> HTIFVQLEADGTTYPVSYGIRTPSYDGPITDVTSNDLACNGGPNPTTPSDKIITVNAGSTVKAIWRHTLTSGADDVMDASHKGPTLAYLKKVDDALTDTGIGGGWFKIQEDGYNNGQWGTSTVITNGGFQYIDIPACIPSGQYLLRAEMIALHAASSTAGAQLYMECAQINIVGGTGGTALPSTTYSIPGIYKATDPGLLVNIYSMSPSSTYTIPGP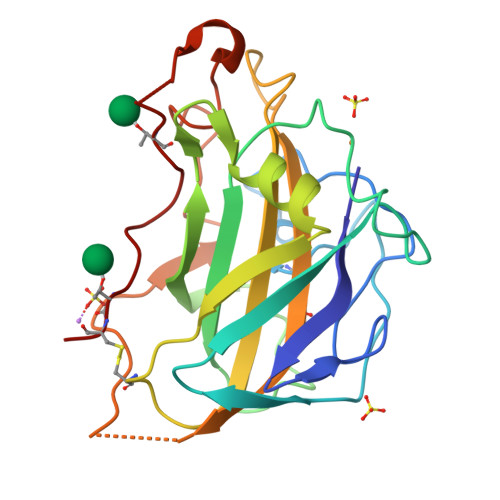AKFTCP>MEQKTLQVEGMSCQHCVKAVETSVGELDGVSAVHVNLEAGKVDVSFDADKVSVKDIA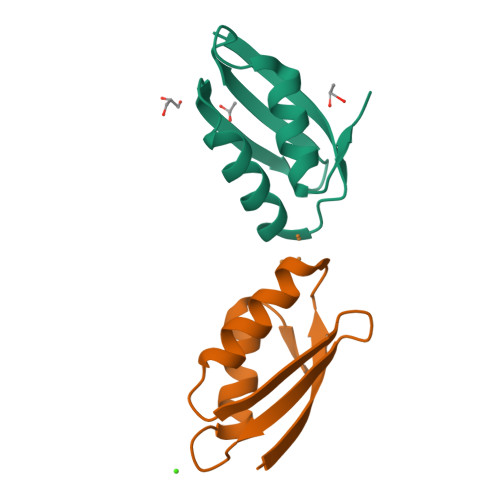DAIEDQGYDVAK[2x]>MQLLLSEAVSRAAKAAGARPLTSPESLSRDLEAPEVQESYRQQLRSDIQKRLQ[4x];>PQVWQLISK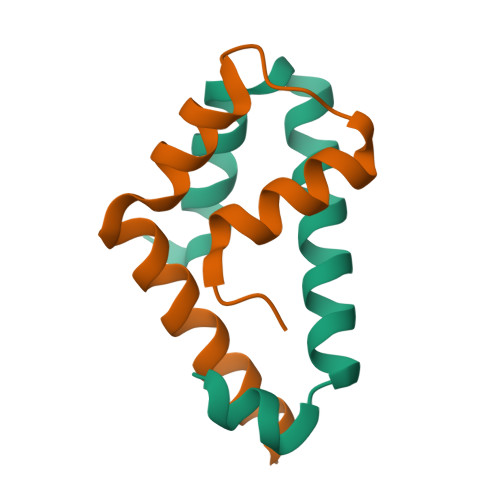VLARHFSAADASRVLEQLQRDYERSLSRLTLDDIERLA[4x]> GMATGDERFYAEHLMPTLQGLLDPESAHRLAVRFTSLGLLPRARFQDSDMLEVRVLGHKFRNPVGIAAGFDK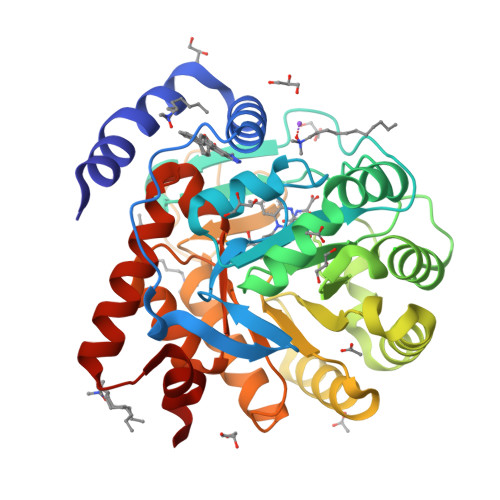HGEAVDGLYKMGFGFVEIGSVTPKPQEGNPRPRVFRLPEDQAVINRYGFNSHGLSVVEHRLRARQQKQAKLTEDGLPLGVNLGKNKTSVDAAEDYAEGVRVLGPLADYLVVNVSSPNTAGLRSLQGKAELRRLLTKVLQERDGLRRVHRPAVLVKIAPDLTSQDKEDIASVVKELGIDGLIVTNTTVSRPAGLQGALRSETGGLSGKPLRDLSTQTIREMYALTQGRVPIIGVGGVSSGQDALEKIRAGASLVQLYTALTFWGPPVVGKVKRELEALLKEQGFGGVTDAIGADHRR>[4x]GADELYRQSLEIISRYLREQATGAKDTKPMGRSGAT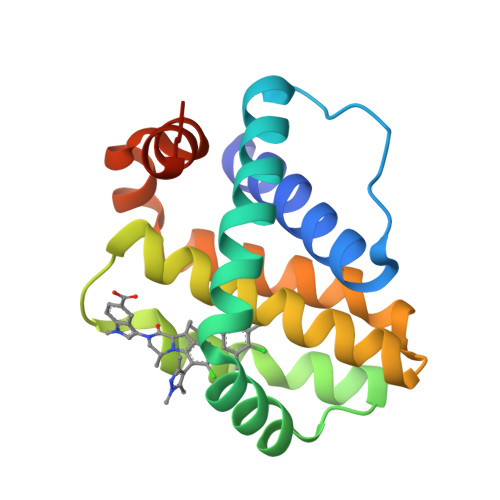SRKALETLRRVGDGVQRNHETAFQGMLRKLDIKNEDDVKSLSRVMIHVFSDGVTNWGRIVTLISFGAFVAKHLKTINQESCIEPLAESITDVLVRTKRDWLVKQRGWDGFVEFFHVEDLEGGI~{tert}-butyl (2'~{S},3~{S})-2-oxidanylidene-2'-propan-2-yl-spiro[1~{H}-indole-3,3'-pyrrolidine]-1'-carboxylate 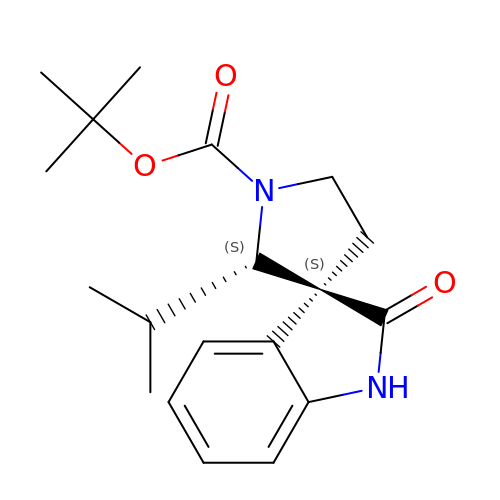| C19 H26 N2 O3 | PENVAQPGQMBKCU-KXBFYZLASA-N> MAATSRPERVWPDGVIPFVIGGNFTGSQRAVFRQAMRHWEKHTCVTFLERTDEDSYIVFTYRPCGCCSYVGRRGGGPQAISIGKNCDKFGIVVHELGHVVGFWHEHTRPDR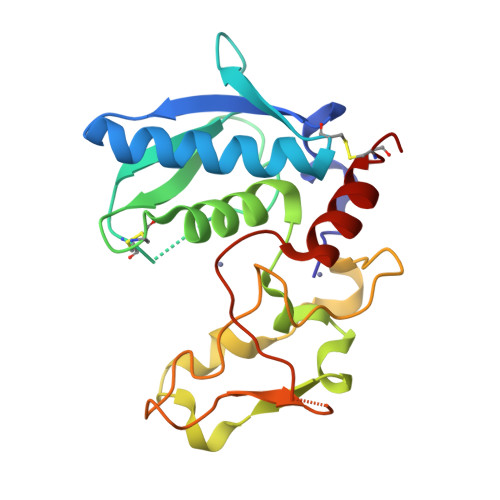DRHVSIVRENIQPGQEYNFLKMEPQEVESLGETYDFDSIMHYARNTFSRGIFLDTIVPKYEVNGVKPPIGQRTRLSKGDIAQARKLYKCPA>[3x]MICLVLTIFANLFPAACTGAH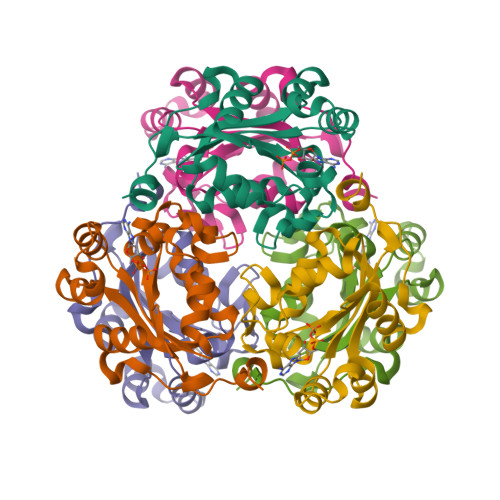ERTFLAVKPDGVQRRLVGEIVRRFERKGFKLVALKLVQASEELLREHYAELRERPFYGRLVKYMASGPVVAMVWQGLDVVRTSRALIGATNPADAPPGTIRGDFCIEVGKNLIHGSDSVESARREIALWFRADELLCWEDSAGHWLYE> MLSYRHSFHAGNHADVLKHTVQSLIIESLKEKDKPFLYLDTHAGAGRYQLGSEHAERTGEYLEGIARIWQQDDLPAELEAYINVVKHFNRSGQLRYYP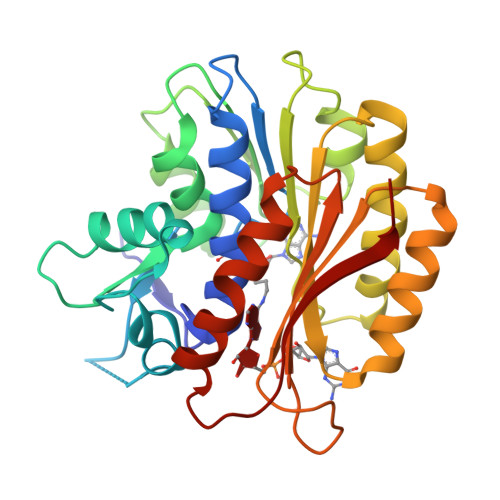GSPLIARQLLREQDSLQLTELHPSDYPLLRSEFQKDSRARVEKADGFQQLKAKLPPVSRRGLILIDPPYEMKTDYQAVVSGIAEGYKRFATGTYALWYPVVLRQQIKRMIHDLEATGIRKILQIELAVLPDSDRRGMTASGMIVINPPWKLEQQMNNVLPWLHSKLVPAGTGHATVSWIVPE>[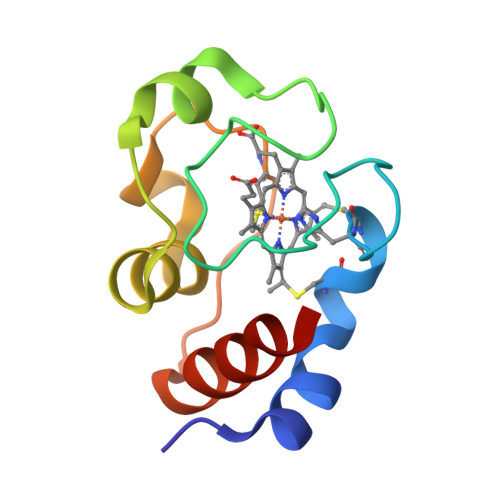3x]EGDAAAGEKAFAPCKACHNFEKNGVGPTLKGVVGAKAGEGADGYAFSDALKKSGLTWDQADLKQWLADPKKKVPGTKMVFPGISDPKKVDDIIAYLKTKS>[2x]MTEDNIAPITSVKVVTDKCTYKDNELLTKYSYENAVVTKTASGRFDVTPTVQDYVFKLDLKKPEKLGIMLIGLGGNNGSTLVASVLANKHNVEFQTKEGVKQPNYFGSMTQCSTLKLGIDAEGNDVYAPFNSLLPMVSPNDFVVSGWDINNADLYEAMQRSQVLEYDLQQRLKAKMSLVKPLPSIYYPDFIAANQDERANNCINLDEKGNVTTRGKWTHLQRIRRDIQNFKEENALDKVIVLWTANTERYVEVSPGVNDTMENLLQSIKNDHEEIAPSTIFAAASILEGVPYINGSPQNTFVPGLVQLAEHEGTFIAGDDLKSGQTKLKSVLAQFLVDAGIKPVSIASYNHLGNNDGYNLSAPKQFRSKEISKSSV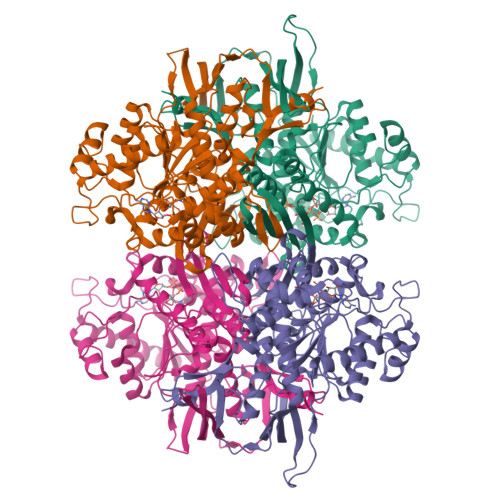IDDIIASNDILYNDKLGKKVDHCIVIKYMKPVGDSKVAMDEYYSELMLGGHNRISIHNVCEDSLLATPLIIDLLVMTEFCTRVSYKKVDPVKEDAGKFENFYPVLTFLSYWLKAPLTRPGFHPVNGLNKQRTALENFLRLLIGLPSQNELRFEERLL> MRTADRKHRVIVCSQQSDVDDEGRLLITRAGVIQGWAAIAPVKAIRFSQDGVSMQKDTMQPTHDITMNYNPDVNVSVSAWVYEHRLKSPPRWFKVLSVVNVDECSRYMKIRCRLVETSDDVTPPVEEEKNSFGAVK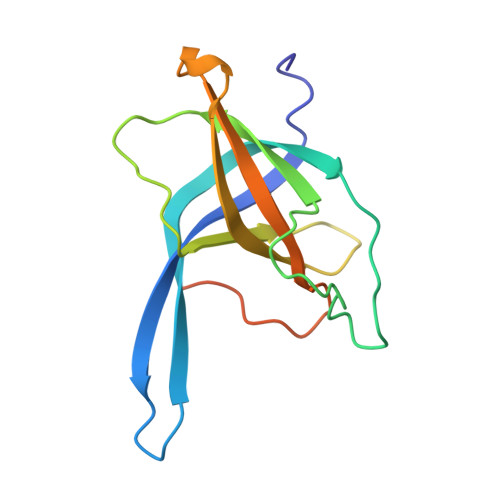IDIPL>MSSGKKPVKVKTPA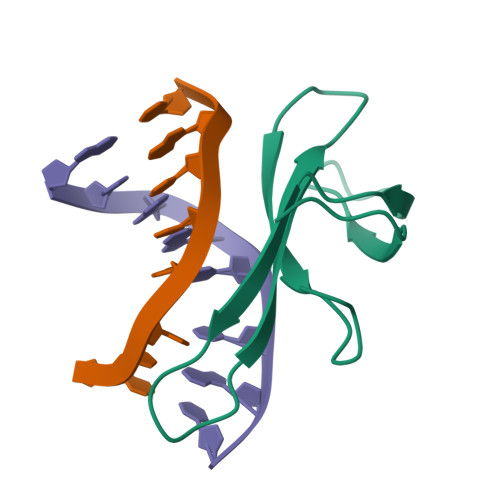GKEAELVPEKVWAFAPKGRKGVKIGLFKDPETGKYFRHKLPDDYPI[2x]6-deoxy-6-(methylamino)-D-galactitol | C7 H17 N O5 | 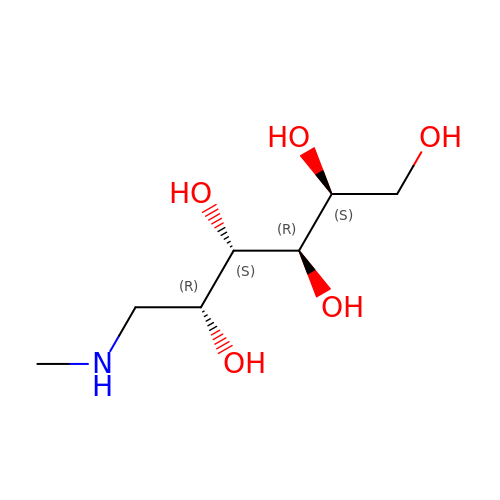MBBZMMPHUWSWHV-JRTVQGFMSA-N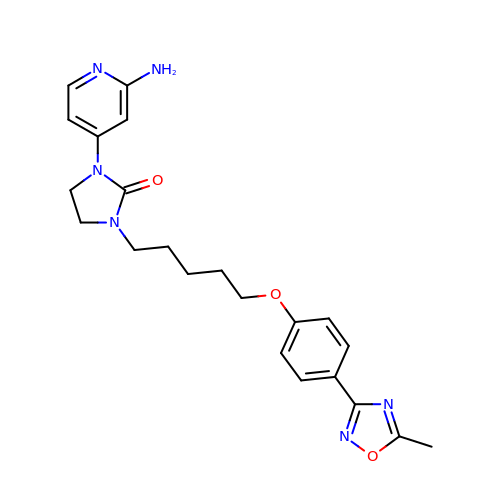1-(2-azanylpyridin-4-yl)-3-[5-[4-(5-methyl-1,2,4-oxadiazol-3-yl)phenoxy]pentyl]imidazolidin-2-one | C22 H26 N6 O3 | HBOHAJJGWJLRSS-UHFFFAOYSA-N> SHIEGYECQPIFLNVLEAIEPGVVCAGHDNNQPDSFAALHSSLNELGERQLVHVVKWAKALPGFRNLHVDDQMAVIQYSWMGLMVFAMGWRSFTNVNSRMLYFAPDLVFNEYRMHKSRMYSQCVRMRHLSQEFGWLQITPQEFLCMKALLLFSIIP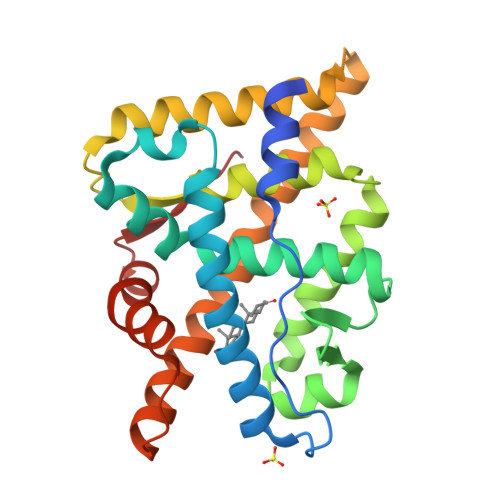VDGLKNQKFFDELRMNYIKELDRIIACKRKNPTSCSRRFYQLTKLLDSVQPIARELYQLTFDLLIKSHMVSVDFPEMMAEIISVQVPKILSGKVKPIYFHTQ pmcAntibiotic resistance mediated by β-lactamase-producing bacteria has become one of the major threats to global health. This phenomenon has substantially reduced the efficacy of β-lactam drugs, which are the most commonly prescribed antibiotics worldwide. β-Lactamases (EC.3.5.2.6) are a group of enzymes that can hydrolyze the amide bond of the β-lactam ring, thus making the antibiotics inactive. One such residue, at position 105 (standard Ambler numbering), is suggested to play an important role in substrate discrimination of class A enzymes. Interestingly, BlaC, the β-lactamase from Mycobacterium tuberculosis, possesses Ile at this position, sparking the question about the evolutionary preference for this amino acid. Mutation of Ile105 to Arg in the β-lactamase BlaC simultaneously enhances activity for carbenicillin and the ability to evade clavulanic acid inhibition.

The crystal structure of BlaC I105R in complex with clavulanic acid revealed the trans-enamine adduct of the inhibitor bound to Ser70 (+155 Da), which is formed after decarboxylation and initial ring opening of the clavulanate. In this complex, residues 105, 130, and 166 are slightly shifted in the I105R enzyme compared to the resting state form. Interestingly, considerably shorter soaking of the wild-type crystal (10 min) was previously found to yield the propionaldehyde ester adduct bound to Ser70 (+70 Da). Although the structural investigation did not indicate any significant repositioning of the active site residues besides 105, we speculate that the larger active site in BlaC I105R causes faster dissociation of the Michaelis complex, thus slowing the initial ring opening of the clavulanate and formation of the acylated species. This is in line with the crystallographic observation that the short soaking of I105R protein crystals with clavulanate (∼10 min) did not yield detectable density for the adduct. The data for wild-type and BlaC I105R could be simulated with values for k2 and k3 that are very similar between wild type and mutant. However, we needed a Ki for I105R that is approximately five times higher than for wild-type, implying that the reduced sensitivity of this variant likely originates from diminished affinity for clavulanic acid, rather than enhanced hydrolysis.

>[2x]DLADRFAELERRYDARLGVYVPATGTTAAIEYRADERFAFCSTFKAPLVAAVLHQNPLTHLDKLITYTSDDIRSRSPVAQQHVQTGMTIGQLCDAAIRYSDGTAANLLLADLGGPGGGTAAFTGYLRSLGDTVSRLDAEEPELNRDPPGDERDTTTPHAIALVLQQLVLGNALPPDKRALLTDWMARNTTGAKRIRAGFPADWKVIDKTGTGDYGRANDIAVVWSPTGVPYVVAVMSDRAGGGYDAEPREALLAEAATCVAGVLA~{N},3-dimethyl-1~{H}-pyrazolo[4,3-d]pyrimidin-7-amine | C7 H9 N5 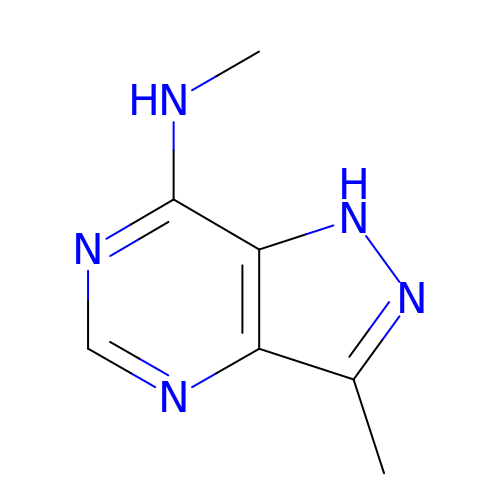| SUUWWTXOJILAMU-UHFFFAOYSA-N> GSHMNGRIYAVGGYDGSPDGHTHLNSVEAYDPETDEWSFVAPMTTPRSGVGVAVLNGRIYAVGGYDGSPDGHTHLNSVEAYDPETDEWSFVAPMTTPRSG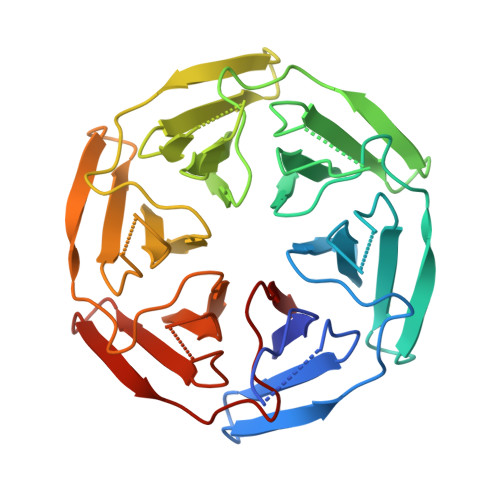VGVAVLNGRIYAVGGYDGSPDGHTHLNSVEAYDPETDEWSFVAPMTTPRSGVGVAVLNGRIYAVGGYDGSPDGHTHLNSVEAYDPETDEWSFVAPMTTPRSGVGVAVLNGRIYAVGGYDGSPDGHTHLNSVEAYDPETDEWSFVAPMTTPRSGVGVAVLNGRIYAVGGYDGSPDGHTHLNSVEAYDPETDEWSFVAPMTTPRSGVGVAVL>SLQPLPPTAFTPNGTYLQHLARDPTSGTLYLGATNFLFQLSPGLQLEATVSTGPVLDSRDCLPPVMPDECPQAQPTNNPNQLLLVSPGALVVCGSVHQGVCEQRRLGQLEQLLLRPERPGDTQYVAANDPAVSTVGLVAQGLAGEPLLFVGRGYTSRGVGGGIPPITTRALWPPDPQAAFSYEETAKLAVGRLSEYSHHFVSAFARGASAYFLFLRRDLQAQSRAFRAYVSRVCLRDQHYYSYVELPLACEGGRYGLIQAAAVATSREVAHGEVLFAAFSSAAPPTVGRPPSAAAGASGASALCAFPLDEVDRLANRTRDACYTREGRAEDGTEVAYIEYDVNSDCAQLPVDTLDAYPCGSDHTPSPMASRVPLEATPILEWPGIQLTAVAVTMEDGHT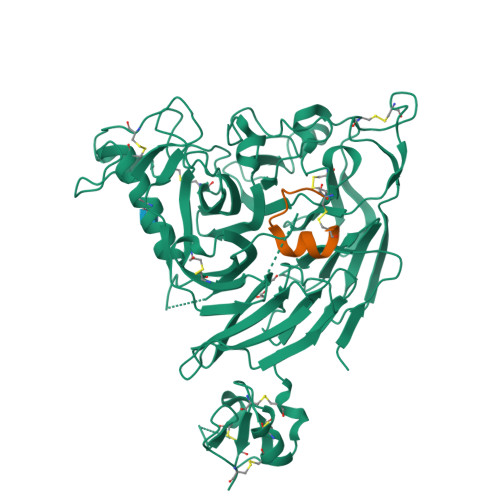IAFLGDSQGQLHRVYLGPGSDGHPYSTQSIQQGSAVSRDLTFDGTFEHLYVMTQSTLLKVPVASCAQHLDCASCLAHRDPYCGWCVLLGRCSRRSECSRGQGPEQWLWSFQPELGCLQTRENLYFQ[2x];>[2x]SEICPSFQRVIETLLMDTPSSYEAAMELFSPDQDMREAGAQLKKLVDTLPQKPRESIIKLMEKIAQSSLSGCNSNVLSWQTYSWYCGSPSFQRVIETLLMDTPSSYEAAMELFSPDQDMREAGAQLKKLVDTLPQKPRESIIKLMEKIAQSSLCN>[3x]GGLEKDFLPLYFGWFLTKKSSETLRKAGQVFLEELGNHKAFKKELRHFISGDEPKEKLELVSYFGKRPPGVL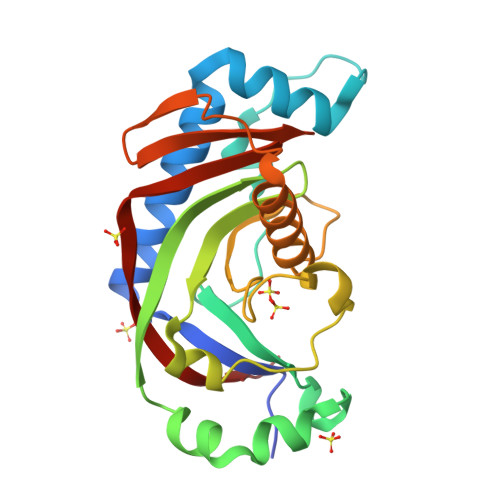HCTTKFCDYGKAAGAEEYAQQEVVKRSYGKAFKLSISALFVTPKTAGAQVVLTDQELQLWPSDLDKPSASEGLPPGSRAHVTLGCAADVQPVQTGLDLLDILQQVKGGSQGEAVGELPRGKLYSLGKGRWMLSLTKKMEVKAIFTGYYG> UUCGC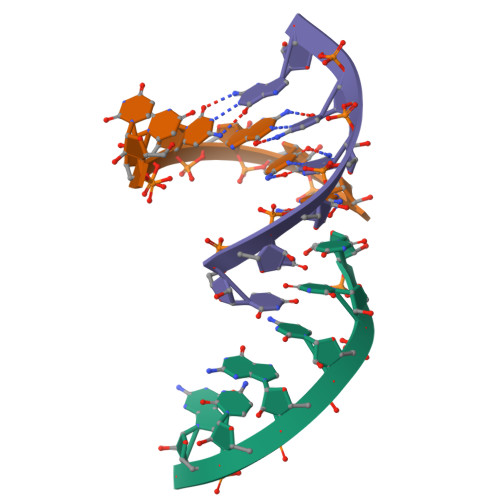G> NSVHPCCDPVKCEPREGEHCISGPCCRNCKFLNAGT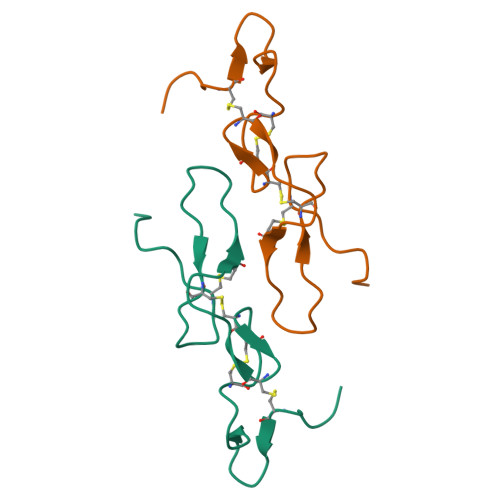ICKRAMLDGLHDYCTGVTSDCPRNRYNH> MKTEWPELVGKSVEEAKKVILQDKPEAQIIVLPVGTIVTMEYRIDRVRIFVDKLDNVAQVPRVG

CI2 is a small single domain protein of 64 residues, which has been extensively used as a model to understand key concepts of protein folding and stability. L49 and I57 are both part of the folding nucleus in CI2 and very important for the stability of the folded state of CI232. Here, we have applied an efficient in-cell assay in E. coli to select variants of the barley chymotrypsin inhibitor 2 with increased stability. We, therefore, determined the crystal structures of all four CI2 variants in the wild-type to L49I/I57V double mutant cycle.

Still, we found two variants, L49I/I57V and D55G, that are significantly stabilized relative to wild-type CI2. For L49I/I57V we find that there is a strong positive synergistic effect between the two substitutions and this variant is stabilized by 5.1 kJ mol−1 more than the sum of the individual effects of the two single variants. Overall, the structures of L49I, I57V and L49I/I57V are highly similar to the structure of the wild-type with RMSDs for the backbone of 0.16, 0.45 and 0.17 Å. Around the mutated residues the structural changes are minimal. The Val at position 57 in I57V and L49I/I57V superimpose, except for the missing δ1 methyl group, with the Ile at position 57 in the wild-type and L49I. In the structure of the double mutant, however, we observe that the Ile at position 49 is found in two alternative conformations. The minor conformation, accounting for roughly 30% of the electron density, has a conformation similar to that seen in L49I. In the major conformation that accounts of the remaining 70% of the electron density, the γ2 methyl is rotated approximately 120° and points towards the position where the δ1 methyl group of the Ile at position 57 would be in the wild-type structure. Although we see small structural changes in the structure compared with the other structures in the mutant cycle, the presence of two distinct conformations of the Ile at position 49 in the double mutant could point to effects of conformational entropy or conformational changes also contributing.>MAVPFVEDWDLVQTLGEGAYG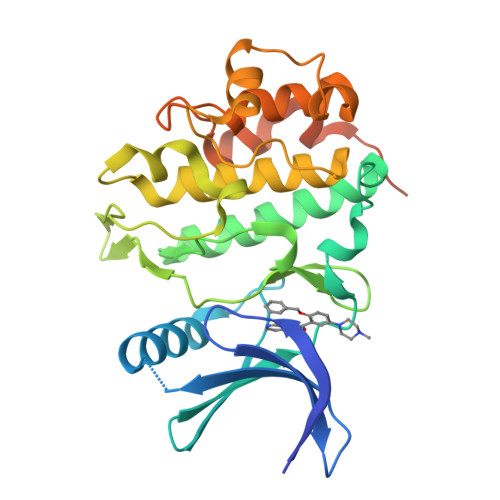EVQLAVNRVTEEAVAVKIVDMKRAVDCPENIKKEICILKMLNHENVIKFYGHRREGNIQYLFMELASGGSLFDRIEPDIGMPEPDAQRFFHQLMAGVVYLHGIGITHRDIKPHNLLLDERDNLKIADFGLATVFRYNNRERLLNKMCGTLPYVAPELLKRREFHAEPVDVWSCGIVLTAMLAGELPWDQPSDSCQEYSDWKEKKTYLNPWKKIDSAPLALLHKILVENPSARITIPDIKKDRWYNKPLKKGAKRPRVTSGGVSESPSGHHHHHHHH[2x]> PDVVLVNGGEPPNPLIPTGTNDSNGGRIIDRLFAGLMSYDAVGKPSLEVAQ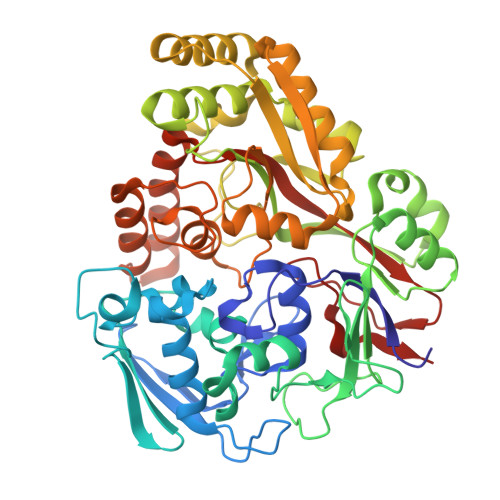SIESADNVNYRITVKPGWKFTDGSPVTAHSFVDAWNYGALSTNAQLQQHFFSPIEGFDDVAGAPGAASRTTMSGLRVVNDLEFTVRLKAPTIDFTLRLGHSSFYPLPDSAFRDMAAFGRNPIGNGPYKLADGPAGPAWEHNVRIDLVPNPDYHGNRKPRNKGLRFEFYANLDTAYADLLSGNLDVLDTIPPSALTVYQRDLGDHATSGPAAINQTLDTPLRLPHFGGEEGRLRRLALSAAINRPQICQQIFAGTRSPARDFTARSLPGFDPNLPGNEVLDYDPQRARRLWAQADAISPWSGRYAIAYNADAGHRDWVDAVANSIKNVLGIDAVAAPQPTFAGFRTQITNRAIDSAFRAGWRGDYPSMIEFLAPLFTAGAGSNDVGYINPEFDAALAAAEAAPTLTESHELVNDAQRILFHDMPVVPLWDYISVVGWSSQVSNVTVTWNGLPDYENIVKA>GTKQEKTALNMARYIRSQTLTLLEKLNELDADEQADICESLHDHADELYRSCLARFGDDGENL[3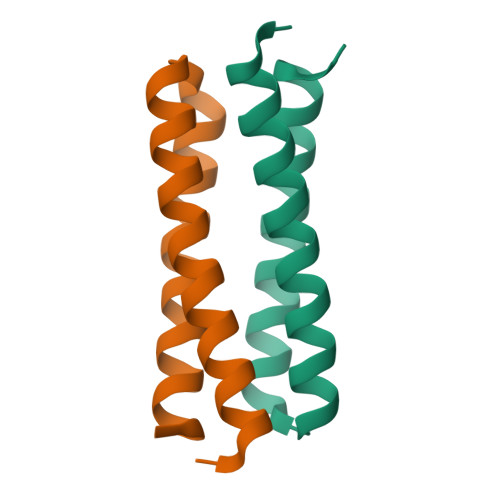x]>[2x]MLQKLIQILRRNEYVKNVYKNTVSNFIETSIPEITPFNARTSSIKGKRLNLLVPSINQEHMFGGISTALKLFEQFDNAAFAKRIILTDATPNPKDLQSFKSFKYVMPEEDKDFALQIVPFNDRYNRTIPVAKHDIFIATAWWTAYAAQRIVSWQSDTYGIPPNKILYIIQDFEPGFYQWSSQYVLAESTYKYRGPQIAVFNSELLKQYFNNKGYNFTDEYFFQPKINTTLKNYINDKRQKEKIILVYGRPSVKRNAFTLIVEALKIFVQKYDRSNEWKIISVGEKHKDIALGKGIHLNSLGKLTLEDYADLLKRSSIGISLMISPHPSYPPLEMAHFGLRVITNKYENKDLSNWHSNIVSLEQLNPENIAETLVELCMSFNNRDVDKKESSNMMFYINEFNEFSFIKEIEEKL

WsaF is the first rhamnosyltransferase to be structurally and biochemically characterised. WsaE is a multifunctional enzyme forming both an α-1,2- and the α-1,3-linkage; WsaF is a β-1,2-rhamnosyltransferase. Both enzymes utilise dTDP-β-l-rhamnose (dTDP-β-l-Rha) as the donor molecule. In the CAZy database, WsaF is annotated to GT4 family, which is the largest retaining GT-B fold family with currently 11,446 entries.

The structures of the dTDP-WsaFSER2 and dTDP-β-l-Rha-WsaFSER2 complexes were obtained by soaking and solved by molecular replacement using SeMet-WsaF as model. The majority of residues that interact with dTDP are located in the C-terminal domain, with the thymidine moiety forming polar interactions with the side chain of K302 and the main-chain atoms of L303 (with O2, N3, and O4 of thymidine). Upon binding of dTDP (or dTDP-β-l-Rha), the side chain of K302 becomes ordered and the amine forms a hydrogen bond with O2 of thymidine. Y308 π stacks (distance 3.9–4.2 Å) with the pyrimidine ring of the dTDP, a common feature in nucleotide binding proteins. E333 hydrogen bonds with the O3 of the 2-deoxyribose. In the dTDP complex, both phosphates make salt links (3.4 Å) with R249, the α-phosphate makes a salt link with K302 (4 Å), and the β-phosphate makes a salt link with R254 (4.2 Å), which has a slightly different conformation as compared to the other structures. Overall, the loop between P325 and P329 changes the conformation slightly upon binding of dTDP. The side chain of H326 turns into the catalytic site. The side chain of N201 shifts in the dTDP complex structure following H326. The dTDP shows interactions with R249, K302, and Y247, all of which are shown by mutagenesis to be important or critical for enzyme function.>[32x]MSIVTKSIVNADAEARYLSPGELDRIKAFVTGGAARLRIAETLTGSRETIVKQAGDRLFQKRPDIVSPGGNAYGEEMTATCLRDMDYYLRLVTYGVVSGDVTPIEEIGLVGVREMYRSLGTPIEAVAQSVREMKEVASGLMSSDDAAEASAYFDFVIGKMS;>[34x]MQDAITAVINSADVQGKYLDGAAMDKLKSYFASGELRVRAASVISANAATIVKEAVAKSLLYSDVTRPGGNMYTTRRYAACIRDLDYYLRYATYAMLAGDASILDERVLNGLKETYNSLGVPISSTVQAIQAIKEVTASLVGADAGKEMGVYLDYICSGLS;>MSVVSQVILQADDQLRYPTSGELKGIQAFLTTGAQRIRIAETLAENEKKIVDQAQKQLFKKHPEYRAPGGNAYGQRQYNQCLRDYGWYLRLVTYGVLAGNKEPIETTGLIGVKEMYNSLNVPVPGMVDAVTVLKDAALGLLSAEDANETAPYFDYIIQFMS[2x];>MRDAVTTLIKNYDLTGRYLDRNAMDELKAYFESGSARIAAAAMINANSATIVKRAAAQLFEEIPELIRPSGNAYTTRRFSACLRDMDYYLRYASYALIAADNNVLDERVLQGLRETYNSLGVPIGPTVRGIQIMKEMIEAMAEDSSLNSTDFIASPFDHMTRELSELSV[2x];>MRMFRITACVPSQTRIRTQRELQNTYFTKLVPYDNWFREQQRIMKMGGKIVKVELATGRPGTNAGLA[6x];>[2x]MSVKASGGSSLARPQLYQTVPVSAISQAEQQDRFLEGSELNELTAYFQSGALRLEIAETLTQNADLIVSRAANRIFTGGSPLSYLEKPVERQPALVGASSDSRNGSVTYAESNGSGGLFGGLRSVFSSTGPIPPGFRPINIARYGPSNMQKSLRDMSWFLRYTTYAIVAGDPNIIVVNTRGLKEVIENACSIDATIVAIQEMRAASADYFRNNAQAKEIVLQYFDILLSEFKAPTPANKVRQGPSNDIQGLELPQSYFNAA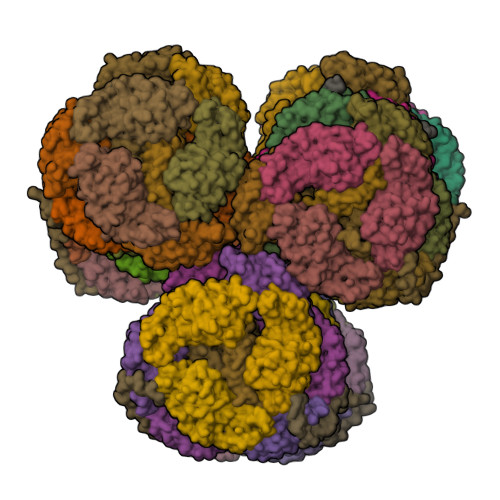AKRQKYAMKPGLSALEKNAVIKAAYRQIFERDITKAYSQSISYLESQVRNGDISMKEFVRRLAKSPLYRKQFFEPFINSRALELAFRHILGRGPSSREEVQKYFSIVSSGGLPALVDALVDSQEYADYFGEETVPYLRGLGVEAQECRNWGMQQDLFSYSAPFRKVPQFITTFAQYDRPLPDQHVYGSGNDPLEIQFGAIFPKETRNPSKRPAPFNKDTKRILIHRGPAVNNQVGNPSAVGEFPGSLGAKVFRLNGGLPGAKVGKNTGTSVKFGESSTQALIRAAYRQVFGRDLYEGQRLSVAEIQLENGDISVREFIKRLAKSELFLKLYWAPHYVCKAIEYMHRRLLGRPTYGRQEMNQYFDIASKQGFYAVVEAMIDSKEYSDAFGEDTVPYERYLTPGGLQMRSARVGSLREDIGQRVDKEVTPRFVELGQVSAIRTEPEIAYRSNQGVTRQRQQTKVFKLVSTYDKVAVKNAIRAAYRQVFERDLEPYIINSEFTALESKLSNNEINVKEFIEGLGTSELYMKEFYAPYPNTKVIEMGTKHFLGRAPLNQKEIQQYNQILASQGLKAFIGAMVNGMEYLQTFGEDTVPYRRFPTLPAANFPNTERLYNKLTKQDKELVVPSFTPVVKVGG;>[6x]MALPLLNYAPKSQNVRVEGYEIGSEEKPVVFTTENILSSSDMDNLIEAAYRQIFFHAFKWDREKVLESQLRNGQITVRDFVRGLLLSNTFRNSFYEKNSNYRFVEHCVQKILGRDVYSEREKIAWSIVVATKGYQGLIDDLLNSDEYLNNFGYDTVPYQRRRNLPGREAGELPFNIKSPRYDAYHRRQLGFPQIVWQNEVRRFIPQEKKLTAGNPMNFLGMARSINPAANTIPKVSAQNINIEASVPRR;>[2x]MLKKLFGAKKEFYVQLDESQAPAQVEEADVAIVKSEVAPVEKPAPTTSKKTSIKKKSATKAAAPVETPASAPVAPAPKAKVDPSQVAFASGDPIPQNVARRTPGPSLNRFKEMARQVKVKR>HTRM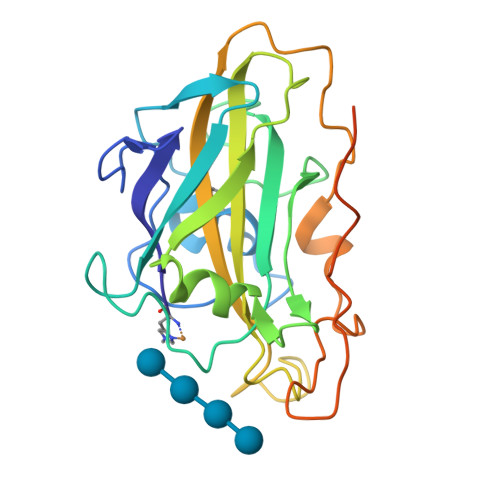FSVWVNGVDQGDGQNVYIRTPPNTDPIKDLASPALACNVKGGEPVPQFVSASAGDKLTFEWYRVKRGDDIIDPSHSGPITTWIAAFTSPTMDGTGPVWSKIHEEGYDASTKSWAVDKLIANKGMWDFTLPSQLKPGKYMLRQEIVAHHESDATFDKNPKRGAQFYPSCVQVDVKGVGGDAVPDQAFDFNKGYKYSDPGIAFDMYTDFDSYPIPGPPVWDAQDEGCCFIDGVDTTSVKEVVKQIICVLK[2x]The most well-studied baculovirus is Autographa californica multiple nucleopolyhedrovirus (AcMNPV). Baculoviruses have their large circular dsDNA genome packaged into an enveloped rod-shaped nucleocapsid. The BV nucleocapsid structure consists of three parts, a central helical sheath containing the viral genome, an apical cap and a basal structure attached to both extremities of the helical sheath. Herein, we report high-resolution cryo-electron microscopy (cryo-EM) structures of the BV nucleocapsid combined with de novo modeling and Alphafold predictions.

The BV apical cap displays a prominent crown-like structure sitting right above the C2 symmetric part of the BV portal, adopting a C21 symmetry and being the vertex of the apical cap. It has a maximum and minimum diameter of 23 and 10 nm respectively. The asymmetric unit of the C21 ring observes a distinctive ‘sickle’ shape, characterized by a straight vertical ‘handle’ domain, connected to a ‘hook’ domain. Thanks to a higher resolution for this ring structure (3.5 Å), the extensive modeling analysis indicated three different proteins, each one in two copies, contributing to form this crown-like C21 ring. The handle region comprises a dimeric Ac66, spanning N-terminal amino acids 4-75, with the remaining amino acids of Ac66 conspicuously absent in the C21 ring structure. The ‘hook’ portion of the asymmetric unit consists of two sets, each constituted of two proteins: Ac101 and Ac102. The first set, encompassing N-terminal amino acids 29-119 of Ac102 and 2-78 of Ac101, is positioned closer and perpendicular to the handle part of the assembly whereas the second set, including amino acids 54-117 of Ac102 and 2-63 of Ac101, is located at the tip of the hook. Within an asymmetric unit, Ac101 pairs up with Ac102 in a heterodimeric arrangement. The interaction between these two proteins is pervasive, extending intimately across the entire modeled length of both proteins, with a spectacular β-strands pairing forming an intermolecular β-sheet. Ac102 of the first set engages in intermolecular interactions with Ac66 through various polar interactions including a potential salt bridge between the Lys32 of Ac66 with Asp41 of Ac102.

>MQRWPKYGGTDVNTRTVHDLLNTINTMSARIKTLERYEHALREIHKVVVILKPSANTHSFEPDALPALIMQFLSDFAGRDINTLTHNINYKYDYNYPPAPVPAMQPPPPPPQPPAPPQPPYYNNYPYYPPYPFSTPPPTQPPESNVAGVGGSQSLNQITLTNEEESELAALFKNMQTNMTWELVQNFVEVLIRIVRVHVVNNVTMINVISSITSVRTLIDYNFTEFIRCVYQKTNIRFAIDQYLCTNIVTFIDFFTRVFYLVMRTNFQFTTFDQLTQYSNELYTRIQTSILQSAAPLSPPTVETVNSDIVISNLQEQLKRERALMQQISEQHRIANERVETLQSQYDELDLKYKEIFEDKSEFAQQKSENVRKIKQLERSNKELNDTVQKLRDENAERLSEIQLQKGDLDEYKNMNRQLNEDIYKLKRRIESTFDKDYVETLNDKIESLEKQLDDKQNLNRELRSSISKIDETTQRYKLDAKDIMELKQSVSIKDQEIAMKNAQYLELSAIYQQTVNELTATKNELSQVATTNQSLFAENEESKVLLEGTLAFIDSFYQIIMQIEKPDYVPISKPQLTAQESIYQTDYIKDWLQKLRSKLSNADVANLQSVSELSDLKSQIISIVPRNIVNRILKENYKVKVENVNAELLESVAVTSAVSALVQQYERSEKQNVKLRQEFEIKLNDLQRLLEQNQTDFESISEFISRDPAFNRNLNDERFQNLRQQYDEMSSKYSALETTKIKEMESIADQAVKSEMSKLNTQLDELNSLFVKYNRKAQDIFEWKTSMLKRYETLARTTAASVQPNVE[2x];>[2x]MIASINDTDMDTDDNMSQARRNRRNRPPARPSAQTQMAAVDMLQTINTAASQTAASLLINDITPNKTESLKILSTQSVGARSLLEPMQANASTIKLNRIETVNVLDFLGSVYDNTIQVIVTE;>MSAIALYLEINKLRLKIDEPMQLAIWPQLFPLLCDEHQSVQLNTDVLINFMMHVARKSQNTILNNNAAIASQYAAGNADVVAAPASAQPTPRPVINLFARANAAAPAQPSEELINMRRYRNAARKLIHHYSLNSTSSTEYKISDVVMTMIFLLRSEKYHSLFKLLETTFDDYTCRPQMTQVQTDTLLDAVRSLLEMPSTTIDLTTVDIMRSSFARCFNSPIMRYAKIVLLQNVALQRDKRTTLEELLIERGEKIQMLQPQQYINSGTEIPFCDDAEFLNRLLKHIDPYPLSRMYYNAANTMFYTTMENYAVSNCKFNIEDYNNIFKVMENIRKHSNKNSNDQDELNIYLGVQSSNAKRKKY[2x]>DCHLSDMLQQLHSVNASKPSERGLVRQEEAEDPACIPIFWVSKWVDYSDKYGLGYQLCDNSVGVLFNDSTRLILYNDGDSLQYIERDGTESYLTVSSHPNSLMKKITLLKYFRNYMSEHLLKAGANITPREGDELARLPYLRTWFRTRSAIILHLSNGSVQINFFQDHTKLILCPLMAAVTYIDEKRDFRTYRLSLLEEYGCCKELASRLRYARTMVDKLLSSRSASNRLK[2x]

For instance, polo-like kinase 1 (Plk1, a member of five Plks), a validated anticancer target, has a unique exterior surface (polo-box domain, PBD) composed of charged, hydrophobic, and hydrophilic domains whose phosphorylation-dependent protein-protein interactions are crucial in regulating mitotic progression and cell proliferation. A large body of evidence suggests that PBD interacts with phosphoserine/phosphothreonine (pS/pT)-containing motifs, and directs the N-terminal catalytic activity to specific subcellular localizations. The polo-box domain consists of two different binding regions, such as the unique, broader pyrrolidine-binding pocket and the conserved, narrow, Tyr-rich hydrophobic channel, among the three Plk polo-box domains (Plks 1–3), respectively. The N-terminal Pro residue on PLHSpT is crucial in conferring specificity by docking its side chain into a unique hydrophobic core (hereafter called the pyrrolidine-binding pocket), which is surrounded by the Trp414, Phe535, and Arg516 residues.

Therefore, we have generated various N-terminal cyclohexyl-truncated analogues (PL-56, -57, -74, and -75) to study the binding nature of PL-49 with respect to the variation in chain lengths on Plk1 PBD-binding regions. However, the binding affinity of these analogues displayed equal potency (PL-56, -57, -75, and -74) when alkyl tethers were increased from one to eleven by atoms on PL-49. Moreover, in contrast to the previous reports in which the longer alkylphenyl group increased the binding affinity, the N-terminus cyclohexyl methyl moiety on PL-57 was strong enough to attain the observed Plk1 PBD-binding affinity in comparison to PL-74. To determine the binding nature of PL-74, we solved the X-ray co-crystal structure of PL-74 in complex with Plk1 PBD. As expected, when the cyclohexyl moiety at the N-terminal of PL-49 was extended, the resulting PL-74 was directed to the Tyr-rich hydrophobic channel and lost the dual-binding ability. Similar to the previously reported peptide derivatives that were bound to the Tyr-rich hydrophobic channel, the side chain of Tyr481 rotates away from the domain to open the channel. But, in contrast, the position of Tyr481 was parallel to the cyclohexyl moiety because of the closer and deeper hydrophobic binding interactions from the N-terminal substitution on PLHSpTM.>MTSFTIPGLSDKKASDVADLLQKQLSTYNDLHLTLKHVHWNVVGPNFIGVHEMIDPQVELVRGYADEVAERIATLGKSPKGTPGAIIKDRTWDDYSVERDTVQAHLAALDLVYNGVIEDTRKSIEKLEDLDLVSQDLLIAH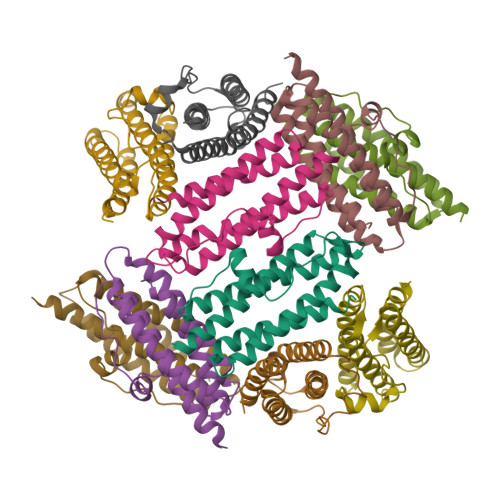AGELEKFQWFVRAHLESAGGQLTHEGQSTEKGAADKARRKSA[10x]> QQKRAFEYEIRFYTGNDPLDVWDRYISWTEQNYPQGGKESNMSTLLERAVEALQGEKRYYSDPRFLNLWLKLGRLCNEPLDMYSYLHNQGIGV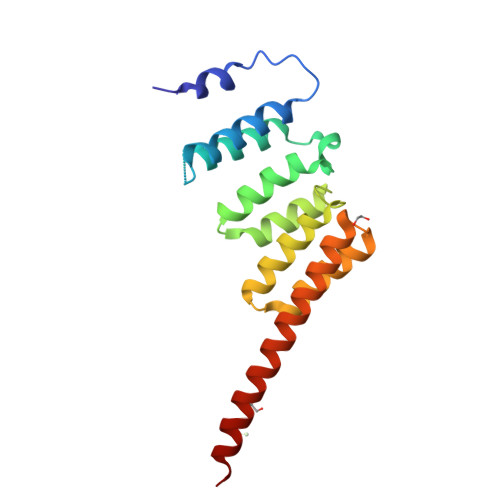SLAQFYISWAEEYEARENFRKADAIFQEGIQQKAEPLERLQSQHRQFQARVSRQTLLALEKEEEEEVFESS>[4x]SNAMKQLTILGSTGSIGNSTLSVVRANPELFKVTALVAGRNVREMAQQCLEFSPRYAAMSDEHSAKSLRLLLAEQGSDTEVYSGETAACELAALD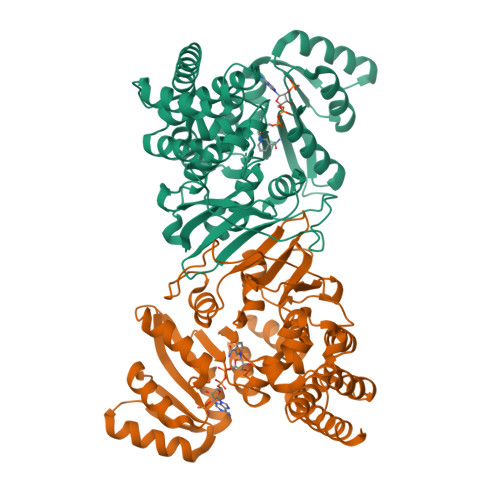DVDQVMAAIVGIAGLPSTLAAIRAGKQVLLANKESLITCGKLFMDEVKRSRAQLLPIDSEHNAIFQSLPERIQRQLGYSSLNENGVSRIILTGSGGPFRETPLSQFSDVTPDQACAHPNWSMGRKISVDSATMMNKGLEYIEARWLFNASAEQIEVVLHPQSVIHSMVRYHDGSILAQMGTPDMRTPIAHAMAYPMRVSSGVAPLDFCKVGALTFTTPDYQRYPCLKLAIDACNAGQAATTALNAANEISVMAFLDSKIRFTDIEVINRTVVEGLLLSEPTSVEEVLVIDRKARDVAAQVIAKLNN> MSLKKVLLCVGNELRGDDGVAIALGRLVEEQMPEWSVFFGYDTPESEFGKLRELAPDVIVVADAMSGFKEGEIEFLDLSDERTYLYSTHNLPTPILISYLRGICSKTIFLGISVLLENV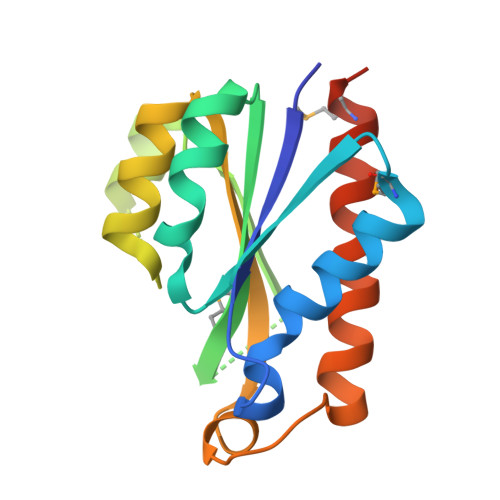LHFSEGLSQGASDSAFVALGRIKELDGMLKEGHHHHHH>SQTKADVVWKDVDGVSMPIPPKTHPRLYLREQQVPDLKNRMNDPKLKKVWADMIKMQEDWKPADIPEVKDFRFYFNQKGLTVRVELMALNYLMTKDPKVGREAITSIIDTLETATFKPAGDISRGIGLFMVTGAIVYDWCYDQLKPEEKTRFVKAFVRLAKMLECGYPPVKDKSIVGHASEWMIMRDLLSVGIAIYDEFPEMYNLAAGRFFKEHLVARNWFYPSHNYHQGMSYLNVRFTNDLFALWILDRMGAGNVFNPGQQFILYDAIYKRRPDGQILAGGDVDYSRKKPKYYTMPALLAGSYYKDEYLNYEFLKDPNVEPHCKLFEFLWRDTQLGSRKPDDLPLSRYSGSPFGWMIARTGWGPESVIAEMKVNEYSFLNHQHQDAGAFQIYYKGPLAIDAGSYTGSSGGYNSPHNKNFFKRTIAHNSLLIYDPKETFSSSGYGGSDHTDFAANDGGQRLPGKGWIAPRDLKEMLAGDFRTGKILAQGFGPDNQTPDYTYLKGDITAAYSAKVKEVKRSFL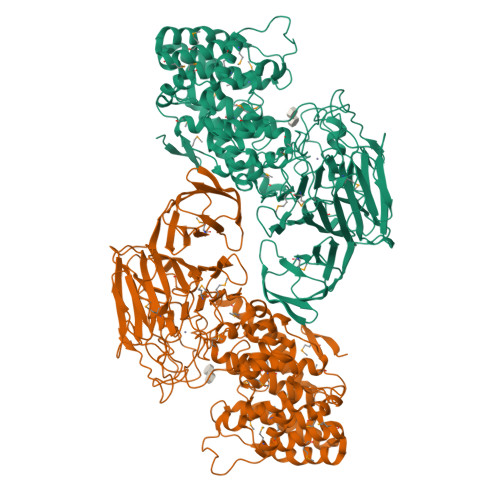FLNLKDAKVPAAMIVFDKVVASNPDFKKFWLLHSIEQPEIKGNQITIKRTKNGDSGMLVNTALLPDAANSNITSIGGKGKDFWVFGTNYTNDPKPGTDEALERGEWRVEITPKKAAAEDYYLNVIQIADNTQQKLHEVKRIDGDKVVGVQLADRIVTFSKTSETVDRPFGFSVVGKGTFKFVMTDLLPGTWQVLKDGKILYPALSAKGDDGALYFEGTEGTYRFLR[2x]>[6x]TRDQNGTWEMESNENFEGYMKALDIDFATRK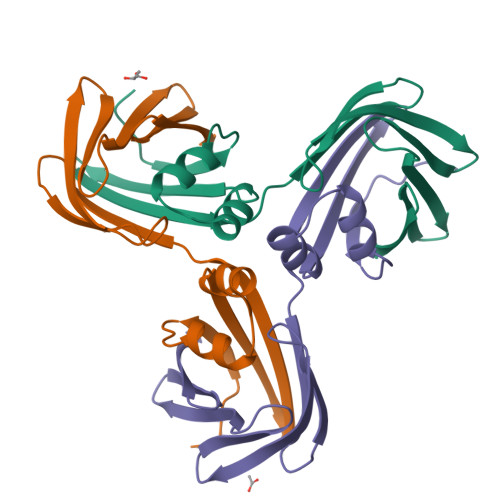IAVRLTQTLVIDQDGDNFKKKTTSTFRNYDVDFTVGVEFDEYTKSLDNRHVKALVTWEGDVLVCVQKGEKENRGWKKWIEGDKLYLELTCGDQVCRQVFKKK> LKHIISAYNFSRDELEDIFALTDKYSKNLNDTRKILSGKTISIAFFEPSTRTYLSFQKAIINLGGDVIGFSGEESTSVAKGENLADTIRMLNNYSDGIVMRHKYD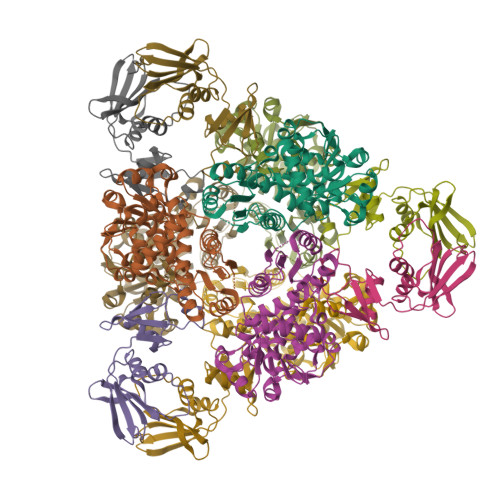GASRFASEISDIPVINAGDGKHEHPTQAVIDIYTINKHFNTIDGLVFALLGDLKYARTVNSLLRILTRFRPKLVYLISPQLLRARKEILDELNYPVKEVENPFEVINEVDVLYVTRIQKERFVDEMEYEKIKGSYIVSLDLANKMKKDSIILHPLPRVNEIDRKVDKTTKAKYFEQASYGVPVRMSILTKIYGE;> MEFMMEIQGNRKELMVSKIKNGTVIDHIPAGRAFAVLNVLGIKGHEGFRIALVINVDSKKMGKKDIVKIEDKEISDTEANLITLIAPTATINIVREYEVVKKTKLEVPKVVKGILKCPNPYCITSNDVEAIPTFKTLTEKPLKMRCEYCETIIDENEIMSQILGANNK>[4x]MAAAAVVAATVPAQSMGADGASSVHWFRKGLRLHDNPALLAAVRGARCVRCVYILDPWFAASSSVGINRWRFLLQSLEDLDTSLRKLNSRLFVVRGQPADVFPRLFKEWGVTRLTFEYDSEPFGKERDAAIMKMAKEAGVEVVTENSHTLYDLDRIIELNGQKPPLTYKRFQALISRMELPKKPAVAVSSQQMESCRAEIQENHDDTYGVPSLEELGFPTEGLGPAVWQGGETEALARLDKHLERKAWVANYERPRMNANSLLASPTGLSPYLRFGCLSCRLFYYRLWDLYKKVKRNSTPPLSLFGQLLWREFFYTAATNNPRFDRMEGNPICIQIPWDRNPEALAKWAEGKTGFPWIDAIMTQLRQEGWIHHLARHAVACFLTRGDLWVSWESGVRVFDELLLDADFSVNAGSWMWLSCSAF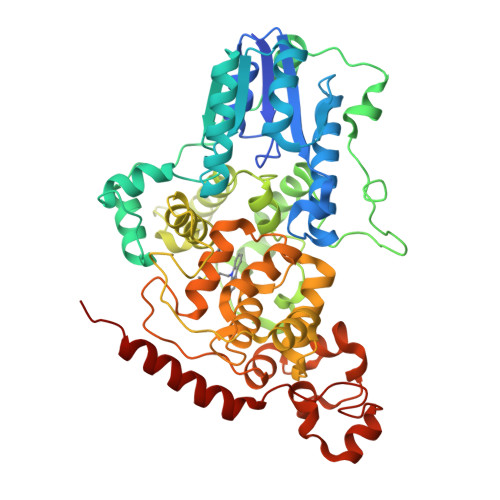FQQFFHCYCPVGFGRRTDPSGDYIRRYLPKLKGFPSRYIYEPWNAPESVQKAAKCIIGVDYPRPIVNHAETSRLNIERMKQIYQQLSRY> SNAMTDAVLELPAATFDLPLSLSGGTQTTLRAHAGHW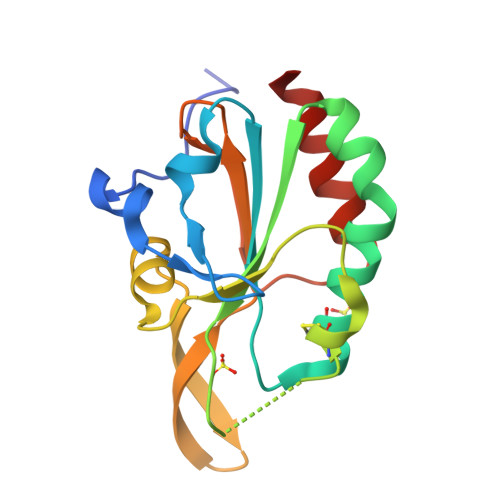LVIYFYPKDSTPGCTTEGLDFNALLPEFDKAGAKILGVSRDSVKSHDNFCAKQGFAFPLVSDGDEALCRAFDVIKEKNMYGKQVLGIERSTFLLSPEGQVVQAWRKVKVAGHADAVLAALKAHAKQ> ALWQFNGMIKCKIPSSEPLLDFNNYGCYCGLGGSGTPVDDLDRCCQTHDNCYKQAMKLDSCKVLVDNPYTNNYSYSCS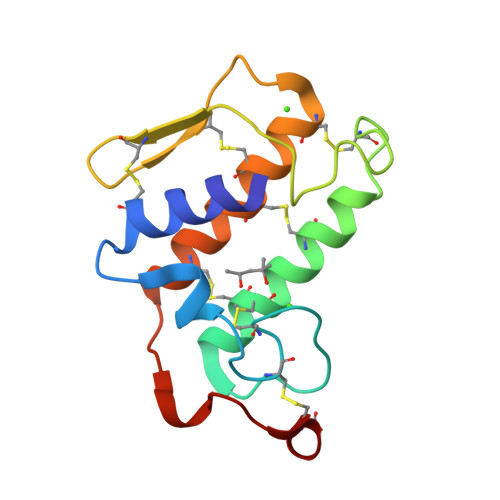NNEITCSSENNACEAFICNCDRNAAICFSKVPYNKEHKNLDMMNC> SKKRQWALEDFEIGRPLGKGKFGNVYLAREKQSKFILALKVLFKAQLEKAGVEHQLRREVEIQSHLRHPNILRLYGYFHDATRVYLILEYAPLGTVYRELQKLSKFDEQRTATYITELANALSYCHSKRVIHRDIKPENLLLGSAGELKIADFGWSVHAPSSRRDTLCGTLDY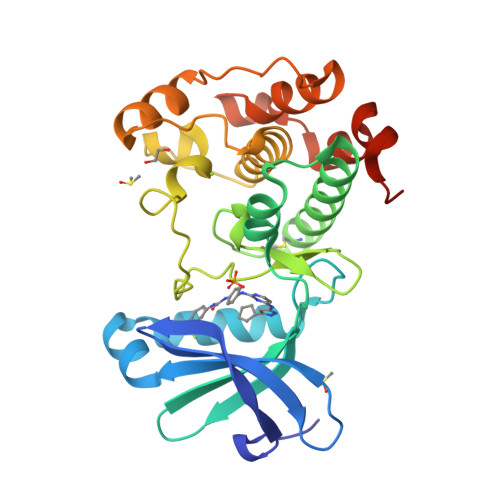LPPEMIEGRMHDEKVDLWSLGVLCYEFLVGKPPFEANTYQETYKRISRVEFTFPDFVTEGARDLISRLLKHNPSQRPMLREVLEHPWITANSSKPSNCQNKESASK1-benzyl-4-(benzylamino)-1H-1,2,4-triazol-4-ium | 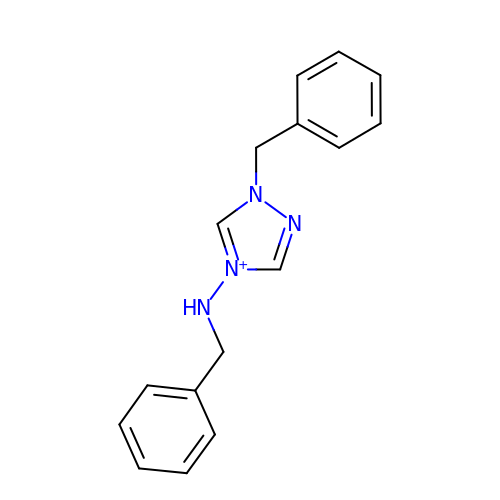C16 H17 N4 | FPCLJFAEMFICTP-UHFFFAOYSA-N>ATIPSESPFAAAEVADGAIVVDIAKMKYETPELHVKVGDTVTWINREAMPHNVHFVAGVLGEAALKGPMMKKEQAYSLTFTEAGTYDYHCTPHPFMRGKVVVE[2x];>EKSKVAGSAAAASAAAASDGSSCDHGPGAISRRSHITLPAYFAGTTENWVSCAGCGVTLGHSLGAFLSLAVAGHSGSDFALASTSFARSAKGKRTDYVEVFDPVTFLPIADIELPDAPRFSVGPRVHIIGNCASSACLLFFLFGSSAAAGLSVPGASDDQLTKSASCFHIHPGAAATHYLGSCPASLAASDLAAAPAAAGIVGAQCTGAQNCSSQAAQANYPGMLVWAVASSILQGDIPAAGATMKAAIDGNESGRKADNFRSAGFQMVAKLKNTDGIMILTVEHSRSCLAAAENTSSVTASVGQTSGPISNGHDSDAIIAAQDGASDNYANSAGTEVLDIYDAASDQDQS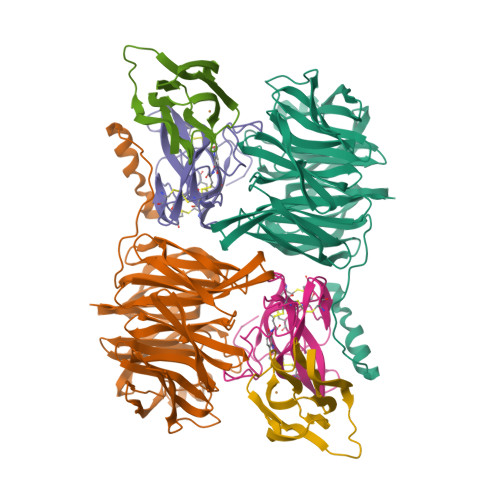SVELDKGPESLSVQNEA[2x];>VDPRAKWQPQDNDIQACDYWRHCSIAGNICDCSAGSLTSCPPGTLVASGSWVGSCYNPPDPNKYITAYRDCCGYNVSGRCACLNTEGELPVYNKDANDIIWCFGGEDGMTYHCSISPVSGA[2x]> MAEAGITGTWYNQLGSTFIVTAGADGALTGTYESAVGNAEGDYVLTGRYDSAPATDGSGTALGWTVAWKNNYRNA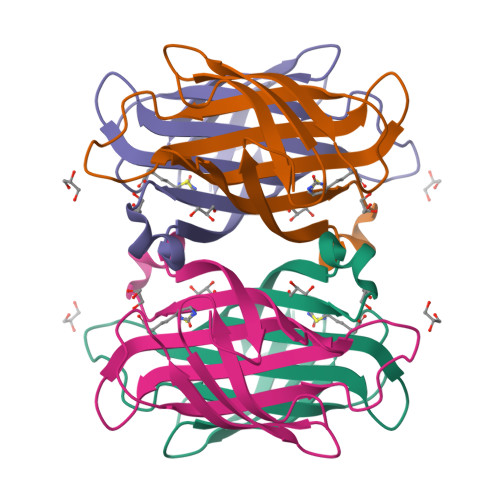HSATTWSGQYVGGAEARINTQWLLTSGTTEANAWKSTLVGHDTFTKVKPSAASHHHHHH> MLTNSEKSRFFLADLTGEVQSIPNTYGYISGLGLFRSAPQTQTTFLMDL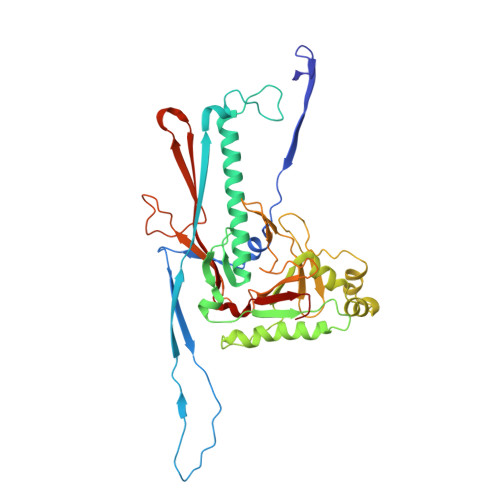TDWDISLLDAVDRTSRKAETSAPERVRQISFPMMYFKEVESITPDEIQGVRQPGTANELTTEAVVRAKKLMKIRTKFDITREFLFMQALKGKVIDANGVLYADLYKQFDVTKKTIYFDLDNPNSDIDAHIEDLRMHMEDEAKTGTVINGEEIHIVVDRTFFSKLIKHPKIRDAYLAQQTPLAWQQITGSLRTGGTDGVQAHMNRFYYGGVVFVQYNGKFKDKRGKTHTLVSIDGVSDTNVGVGHAFPNVAMLGEANNIFEVAYAPCPKMGYANTLGQELYVFEYEKDRDEGIDFEAHSYMLPYCTRPQLLVDVRSDAE>[2x]ALADPLKVMISGAPASGKGTQCELIKTKYQL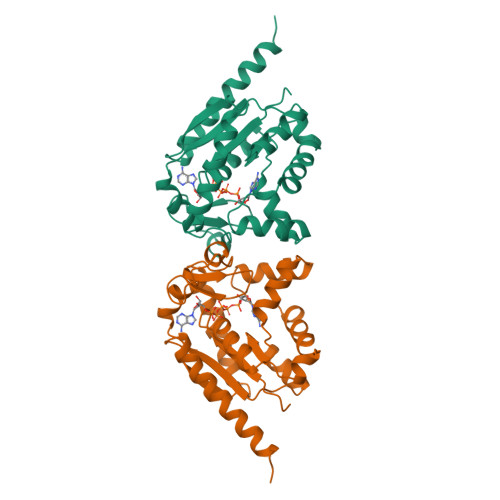AHISAGDLLRAEIAAGSENGKRAKEFMEKGQLVPDEIVVNMVKERLRQPDAQENGWLLDGYPRSYSQAMALETLEIRPDTFILLDVPDELLVERVVGRRLDPVTGKIYHLKYSPPENEEIASRLTQRFDDTEEKVKLRLETYYQNIESLLSTYENIIVKVQGDATVDAVFAKIDELLGSILEKKNEMVSST> MKYFTVFTALTALFAQASASAIPAVRSTLTPRQNTTASCANSATSRSCWGEYSIDTNWYDVTPTGVTREYWLSVENSTITPDGYTRSAMTFNGTVPGPAIIADWGDNLIIHVTNNLEHNGTSIHWHGIRQLGSLEYDGVPGVTQCPIAPGDTLTYKFQVTQYGTTWYHSHFSLQYGDGLFGPLIINGPATADYDEDVGVIFLQDWAHESVFEIWDTARLGAPPALENTLMNGTNTFDCSASTDPNCVGGGKKFELTFVEGTKYRLRLINVGIDSHFEFAIDNHTLTVIANDLVPIVPYTTDTLLIGIGQRYDVIVEANAAADNYWIRGNWGTTCSTNNEAANATGILRYDSSSIANPTSVGTTPRGTCEDEPVASLVPHLALDVGGYSLVDEQVSSAFTNYFTWTINSSSLLLDWSSPTTLKIFNNETIFPTEYNVVALEQTNANEEWVVYVIEDLTGFGIWHPIHLHGHDFFIVAQETDVFNSDESPAKFNLVNPPRRDVAALPGNGYLAIAFKLDNPGSWLLHCHIAWHASEGMAMQFVESQSSIAVKMTDTAIFEDTCANWNAYTPTQLFAEDDSGI

Laccases are members of a large family of multicopper oxidases that catalyze the oxidation of a wide range of organic and inorganic substrates accompanied by the reduction of dioxygen to water. These enzymes contain four Cu atoms per molecule organized into three sites: T1, T2 and T3. The substrate oxidation takes place at the T1 site and molecular oxygen is reduced to water at the T2/T3 site. In this work, the laccase from the ascomycete Botrytis aclada was studied, which contains conserved Ile491 and nonconserved Leu499 residues in the axial positions.

In the present study, we prepared the L499M mutant of the laccase from B. aclada, in which the nonconserved leucine residue in the axial position of the T1 site was replaced by a methionine. The structures of BaL and L499M BaL were solved at 1.67 and 1.7 Å resolution, respectively. The overall structure of L499M BaL is similar to that of BaL and can be superimposed with a Cα r.m.s.d. of 0.10 Å. A comparison of the structures of BaL and L499M BaL shows that there are no changes in the structure of the enzyme except for the region near the axial mutation. In BaL, as in most of the known laccases, the Cu1 ion lies in the plane formed by the coordinated atoms of histidine and cysteine residues. In the T1 site of L499M BaL, Cu1 is displaced from this plane towards the Sδ atom of Met499 by 0.17 Å. In the L499M BaL structure the distance between Cu1 and the Sδ atom of Met499 is 3.2 Å, which also can be ascribed to a weak coordination bond. Hence, the 140 mV decrease in the redox potential of L499M BaL can be attributed exclusively to the mutation. The specific activity of L499M BaL towards ABTS was lower than that of BaL over the whole pH range and was lower for 2,6-DMP at pH < 5, which is consistent with the lower potential of the T1 site of L499M BaL. However, in the pH range 5–7 L499M BaL showed a higher activity than BaL.>[8x]MGSSHHHHHHSSGRENLYFQGMY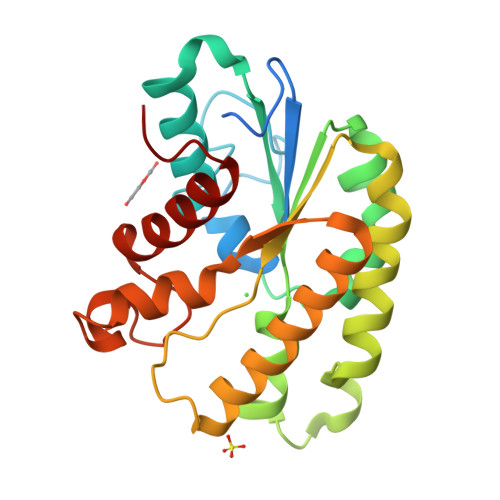FAAGSKLVIIGDSITDAGRDKGIGGEGLFNAHGSGYVALLNAHLFARFPERRLRLVNQGNSGNTVRDLAARWQNDVFGLKPDYVAMMIGINDVWRQFDLPLMTDRHVCPEEYEKTLDELVARTAPTVKGMILLTPYFIEPNREDAMRARMDVYGDLMRRVAERHGCLLVDVQGAFDRYLQHYHPAQLAWDRIHPNLAGHQVIANAFLAATGCLNS> GSHMSPREQDRFLPIANVSRIMKKALPANAKISKDAKETM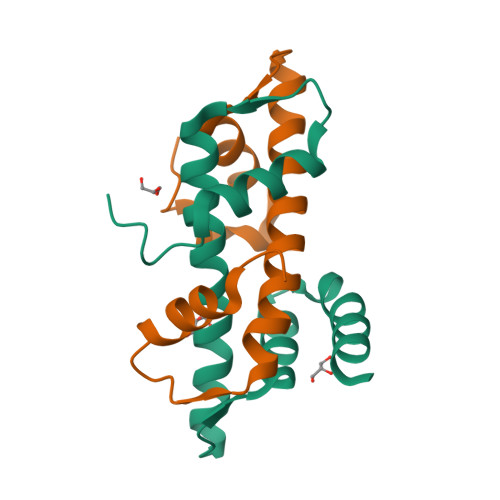QECVSEFISFVTGEASDKCQKEKRKTINGDDLLWAMTTLGFEDYVEPLKVYLQRFRE;> MTQFKEIEKTTDFKNHSLPLARIKKIMKADEDVRMISAEAPVVFARACEMFILELTLRSWNHTEENKRRTLQKNDIAAAVTRTDIFDFLVDIVPR> SLSIEETNKLRAKLGLK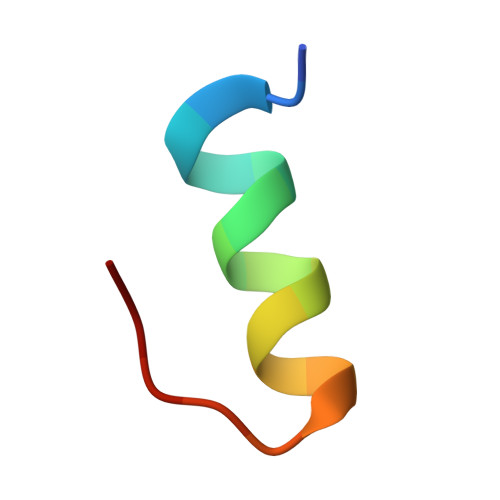PL Substrate-binding proteins (SBPs) are key structural elements of the ABC transporter system that determine the substrate specificity and high affinity of the ABC uptake system. A typical SBP consists of two α/β domains, which are connected by a hinge region. To understand their molecular functions, we performed a crystallographic study of single domain SBP from Rhodothermus marinus (RmSBP). The overall structure of RmSBP showed the single α/β fold, which is identical with that previous reported, although the molecular flexibility was distinct.

The crystal of RmSBP soaked with HgCl2 (RmSBP-Hg) belongs to the monoclinic P21 space group with the unit cell parameters a = 92.84, b = 97.86, c = 101.98 Å, and β = 90°, containing two RmSBP molecules in the asymmetric unit, which is a new crystal form and diffracted up to 2.0 Å. The two RmSBP-Hg molecules in the asymmetric unit clearly showed an electron density map for building all amino acids from Glu27 to Leu182. The crystal structure of RmSBP-Hg showed a strong positive Fo–Fc electron density (>7 sigma) on the Cys145 in the loop between the α5-helix and β5-stand, which surrounds the α5-and α6-helices. Hg2+ interacted with Cys145 and a water molecule at an average distance of 2.57 and 2.27 Å, respectively. Hg2+ was surrounded by Ile122, Thr126, Val132, Val163, and Met167 residues. In the RmSBP-Hg-A molecule, Hg2+ was buried by neighboring amino acids, but in the surface structure of the RmSBP-Hg-B molecule, the conformations of the amino acids around Hg2+ were slightly different, and Hg2+ was observed through the hole in the surface structure. The Cys145 of RmSBP, where Hg2+ bound, was located on the side of the α/β domain, which is different from the previously expected substrate-binding site. The Cys145 with Hg2+ binding in RmSBP is conserved in RpSBP but has been replaced by proline in the other SBPs. This result indicates that Hg2+ may not be directly involved in the biological function of SBP. Accordingly, the mercury associated with RmSBP-Hg is most likely a result of the affinity between Hg2+ and cysteine due to atomic properties, rather than biological function.

>[2x]MHTLRLFTVLSLLLTSAFTLFPETETEVTPIQQLFLIKELKPGIARIGVIWDKNAANRDEVLPQLQRASAATGIKVVVAEVASLQEVAPQFRTLLRDHQVEALWVLEESGLLGQAAARSFLIKNATQAGMPVFAPSETWLKEGACVTWRKDAEGIRLVVNKAVAEAMGITIPAKYQDRTAFLAMN>SIPLIGERFPEMEVTTDHGVIKLPDHYVSQGKWFVLFSHPADFTPVSTTEFVSFARRYEDFQRLGVDLIGLSVDSVFSHIKWKEWIERHIGVRIPFPIIADPQGTVARRLGLLHAESATHTVRGVFIVDARGVIRTMLY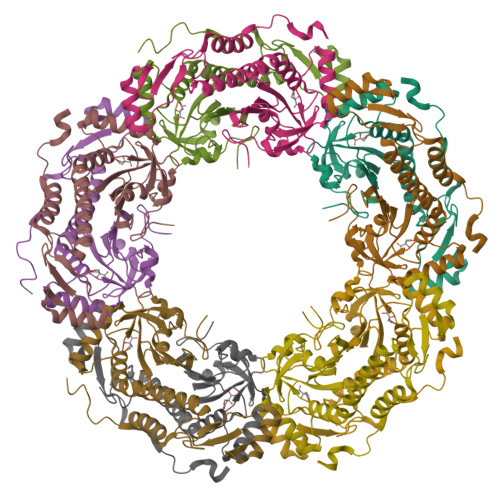YPMELGRLVDEILRIVKALKLGDSLKRAVPADWPNNEIIGEGLIVPPPTTEDQARARMESGQYRSLDWAFSWDTPASRDDVEEARRYLRRAAEKPAKLLYEEA[10x]>[3x]SMGKTLRFEIVSGVNKGYFHTNSQSESLDLVGGIWQKIAKEEFEKSNIYVSAVIKPSKTVYNQEWGCPENGEETVVLTGVANEE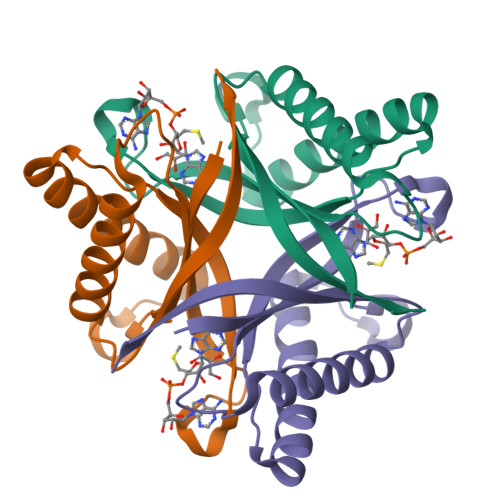FVDDIEKWKDTVIKLAKELKNQMKQSTLTCEFIETELHYFK2',4,4'-TRIHYDROXYCHALCONE | C15 H12 O4 | 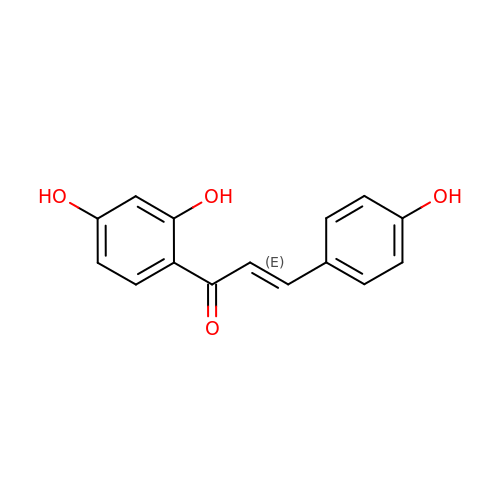DXDRHHKMWQZJHT-FPYGCLRLSA-N> SMSIHRRRTDPMVTLSSILESIINDMRDLPNTYPFHTPVNAKVVKDYYKIITRPMDLQTLRENVRKRLYPSREEFREHLELIVKNSATYNGPKHSLTQISQSMLDLCDEKLKEKE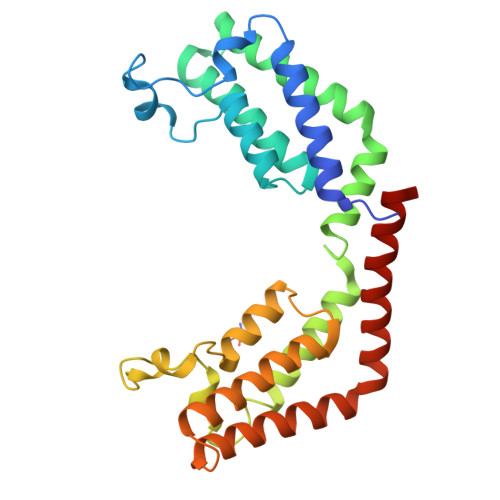DKLARLEKAINPLLDDDDQVAFSFILDNIVTQKMMAVPDSWPFHHPVNKKFVPDYYKVIVNPMDLETIRKNISKHKYQSRESFLDDVNLILANSVKYNGPESQYTKTAQEIVNVCYQTLTEYDEHLTQLEKDICTAKEAALEEAELESLD> HHHHHHSSGLVPRGSHMAIYADNSYSIGNTPLVRLKHFGHNGNVVVKIEGRNPSYSVKCRIGANMVWQAEKDGTLTKGKEIVDATSGNTGIALAYVAAA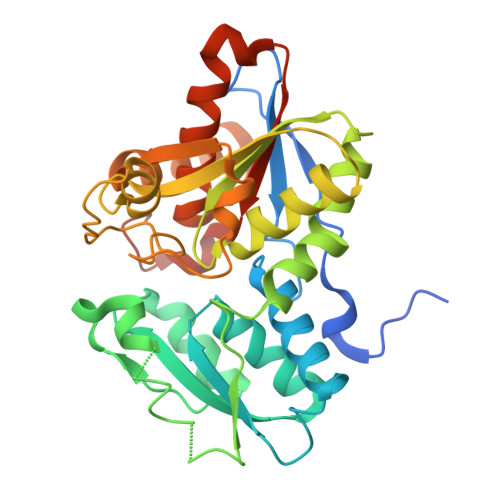RGYKITLTMPETMSLERKRLLCGLGVNLVLTEGAKGMKGAIAKAEEIVASDPSRYVMLKQFENPANPQIHRETTGPEIWKDTDGKVDVVVAGVGTGGSITGISRAIKLDFGKQITSVAVEPVESPVISQTLAGEEVKPGPHKIQGIGAGFIPKNLDLSIIDRVETVDSDTALATARRLMAEEGILAGISSGAAVAAADRLAKLPEFADKLIVVILPSASERYLSTALFEGIEG>MKKEFSAGGVLFKDGEVLLIKTPSNVWSFPKG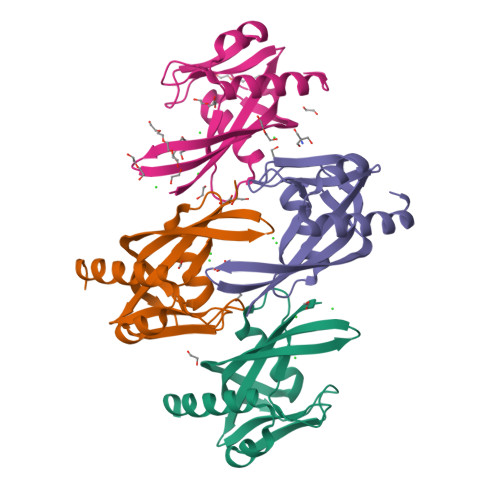NIEPGEKPEETAVREVWEETGVKGEILDYIGEIHYWYTLKGERIFKTVKYYLMKYKEGEPRPSWEVKDAKFFPIKEAKKLLKYKGDKEIFEKALKLKEKFKL[4x]> LDRADILYNIRQTSRPDVIPTQRDRPVAVSVSLKFINILEVNEITNEVDVVFWQQTTWSDRTLAWNSSHSPDQVSVPISSLWVPDLAAYNAISKPEVLT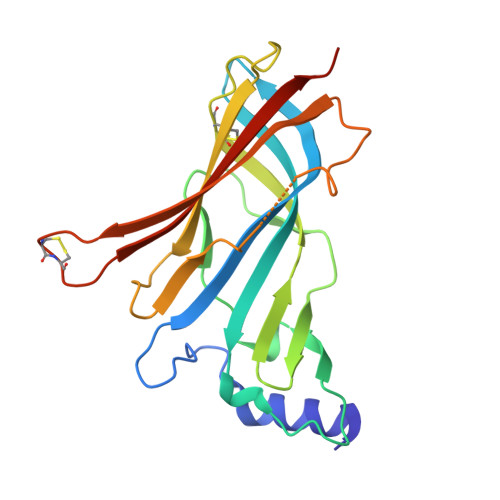PQLARVVSDGEVLYMPSIRQRFSCDVSGVDTESGATCRIKIGSWTHHSREISVDPTTENSDDSEYFSQYSRFEILDVTQKKNSVTYSCCPEAYEDVEVSLNFRKKGRSEIL4,6-dimethylpyrimidin-2-amine 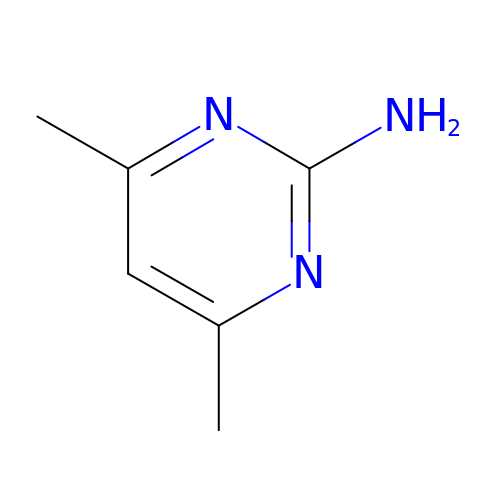| C6 H9 N3 | IDQNBVFPZMCDDN-UHFFFAOYSA-N>MAGGKLTPRQKMINLMYLVFIAMLAMNVSKEVISAFGLMNEKFEAANTSSVTTNESLLTSLDQKAAEAKGEFAKAAETAHKVQAASKEFYDYIGTLKTQAVKGFEVDKETGKMPYEAMDRGDNIDDWFTGDGYTKKGNEIIAKIEKYKSDIKAALGTDKKYAGIISEVEKKFDVSDVKNKEGIKEKYLAYHFKGFPAIASAAKLSAWQNDVKKTEADVYNSALGKAAVAAASYSNYQAIVVLDKNAYFQGEKVTGKVVLGRYDENTKPTSFQGPGQIVNGQAVISLTAGGVGEQDINGQFTFLEDGKNIPLKFSGKYVVVPRPNSATISADKMNVVYRGVVNPISVSFAGVDANKIVASAPGLSSAGKPGKYNMSPGQGTEATISVTGTLPNGDKVTDKKTFRIKGIPGPTGTIRGEMGVVKGPKSNLEIATIGAKLLDFDFEVGLDVVGFNMKIAGQPTVVVTGNKMNAQCKSVLARAGKGDQVTISEIKTKLVGAGSYLLPRTAPVIYEIQ[2x];>[5x]MALLSKKVMNFAYGMGAAVVIVGALFKITHFEIGPLTGTVMLSIGLLTEALIFALSAFEPVEDELDWTLVYPELANGQARKKEAKAETATDAQGLLSQKLDAMLKEAKVDGELMASLGNSIKNFEGAAKAISPTVDSIAGQKKYAEEMS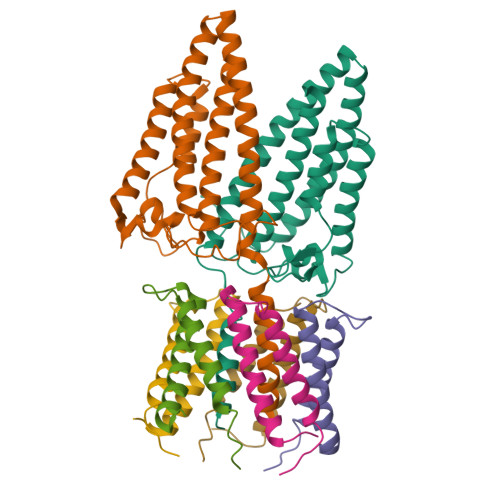MAAAQMESLNSLYKVQLESASRNAQANSEIAENAAKLKEQMASMTANIASLNSVYGGMLSAMSNKG> MANLHILSKLQE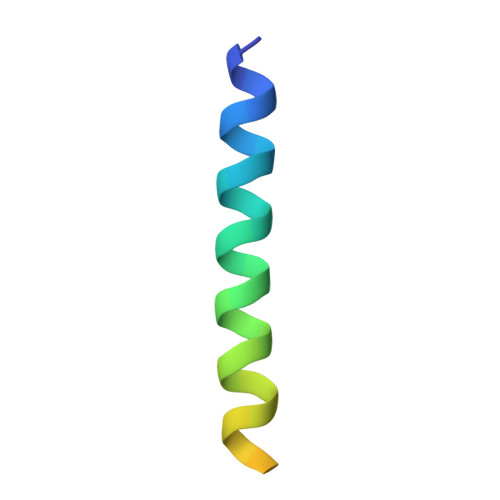EMKRLAEEREETRHGGSRGDMLEVLFQ>[2x]MPPQLHNGLDFSAKVI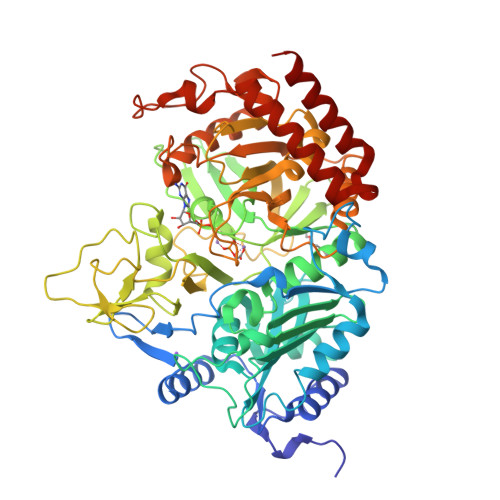QGSLDSLPQEVRKFVEGNAQLCQPEYIHICDGSEEEYGRLLAHMQEEGVIRKLKKYDNCWLALTDPRDVARIESKTVIITQEQRDTVPIPKSGQSQLGRWMSEEDFEKAFNARFPGCMKGRTMYVIPFSMGPLGSPLAKIGIELTDSPYVVASMRIMTRMGTSVLEALGDGEFIKCLHSVGCPLPLKKPLVNNWACNPELTLIAHLPDRREIISFGSGYGGNSLLGKKCFALRIASRLAKEEGWLAEHMLILGITNPEGKKKYLAAAFPSACGKTNLAMMNPTLPGWKVECVGDDIAWMKFDAQGNLRAINPENGFFGVAPGTSVKTNPNAIKTIQKNTIFTNVAETSDGGVYWEGIDEPLAPGVTITSWKNKEWRPQDEEPCAHPNSRFCTPASQCPIIDPAWESPEGVPIEGIIFGGRRPAGVPLVYEALSWQHGVFVGAAMRSEATAAAEHKGKVIMRDPFAMRPFFGYNFGKYLAHWLSMAHRPAAKLPKIFHVNWFRKDKNGKFLWPGFGENSRVLEWMFGRIEGEDSAKLTPIGYVPKEDALNLKGLGDVNVEELFGISKEFWEKEVEEIDKYLEDQVNADLPYEIERELRALKQRISQM>MDSKLIGKICKSIRYRDYETAIFLAACLLPCKPEYRMLMSIVLYLNGEYTRALFHLHKLNTCTSKYYESLCYKKKKDYKKAIKSLESILEGKVERDPDVDARIQEMFVDPGDEEFFESLLGDLCTLSGYREEGIGHYVRSFGKSFLFSPVENLLLENKVPQKRDKENVRQTGRRG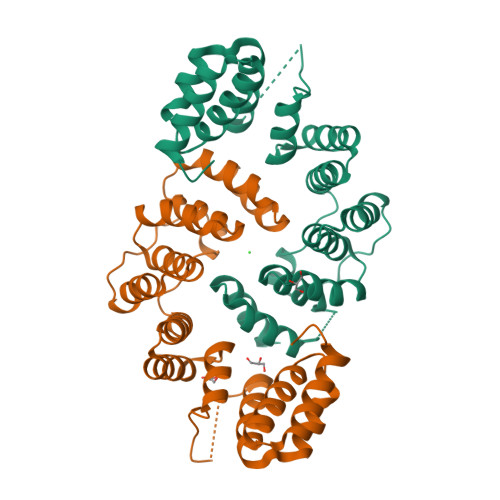IEEEYVSDSIEFHESLSPSLVKKYMEHVPGIGSYFISNAARRYFNLGMNDKSKACFELVRRKDPMFL[4x]> GGGAAPTETQPPVTNLSVSVENLCTVIWTWNPPEGASSNCSLWYFSHFGDKQDKKIAPETRRSIEVPLNERICLQVGSQCSTNESEKPSILVEKCISPPEGDPESAVTELQCIWHNLSYMKCSWLPGRNTSPDTNYTLYYWHRSLEKIHQCENIFREGQYFGCSFDLTKVKDSSFEQHSVQIMVKDNAGKI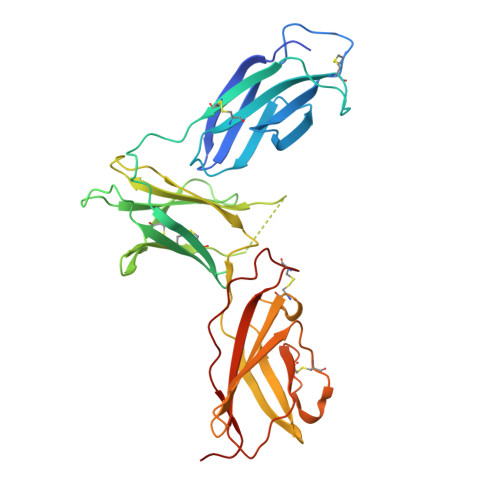KPSFNIVPLTSRVKPDPPHIKNLSFHNDDLYVQWENPQNFISRCLFYEVEVNNSQTETHNVFYVQEAKCENPEFERNVENTSCFMVPGVLPDTLNTVRIRVKTNKLCYEDDKLWSNWSQEMSIGKKR>MEYGPIPSSKFTDVIHHLRHNFPDEPLNASVGLCVHGKPCELLEHHDLQTLEDGLSIMAVESTTGEIAGVALNGIARRGDVEKALEEMKSIDNIKYQRIFGLLNNVNKSIDLFTKYNVDKIFELRILSVDSRFRGRGIAKELFLRSELIAEEHGFKLVKVDATSLFTQRAAECLGFITEKCVTYGDF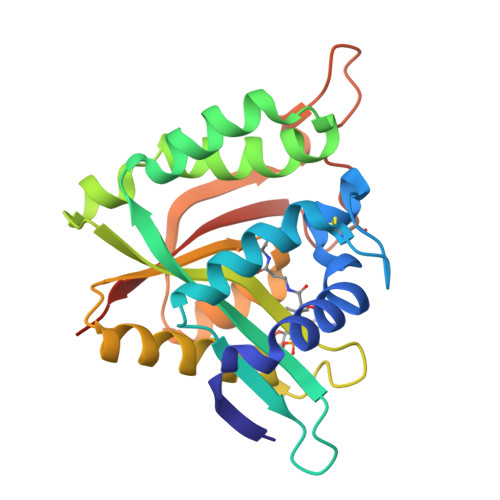KDENGRKIYDTKSPHDYYKVMTKVVSPKSNDG[6x]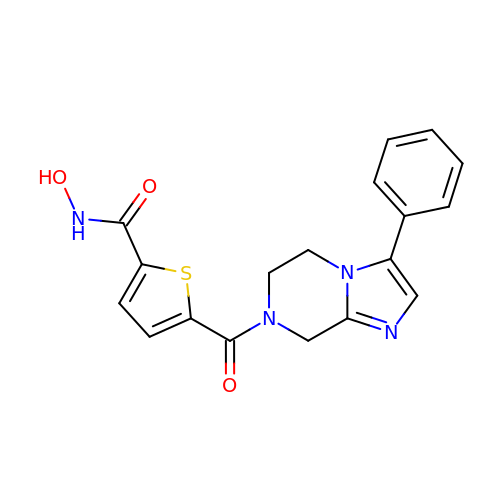N-hydroxy-5-[(3-phenyl-5,6-dihydroimidazo[1,2-a]pyrazin-7(8H)-yl)carbonyl]thiophene-2-carboxamide | C18 H16 N4 O3 S | SMSIXMLQOONOQQ-UHFFFAOYSA-N> MGSDLVLGLDIGIGSVGVGILNKVTGEIIHKNSRIFPAAQAENNLVRRTNRQGRRLARRKKHRRVRLNRLFEESGLITDFTKISINLNPYQLRVKGLTDELSNEELFIALKNMVKHRGISYLDDASDDGNSSVGDYAQIVKENSKQLETKTPGQIQLERYQTYGQLRGDFTVEKDGKKHRLINVFPTSAYRSEALRILQTQQEFNPQITDEFINRYLEILTGKRKYYHGPGNEKSRTDYGRYRTSGETLDNIFGILIGKCTFYPDEFRAAKASYTAQEFNLLNDLNNLTVPTETKKLSKEQKNQIINYVKNEKAMGPAKLFKYIAKLLSCDVADIKGYRIDKSGKAEIHTFEAYRKMKTLETLDIEQMDRETLDKLAYVLTLNTEREGIQEALEHEFADGSFSQKQV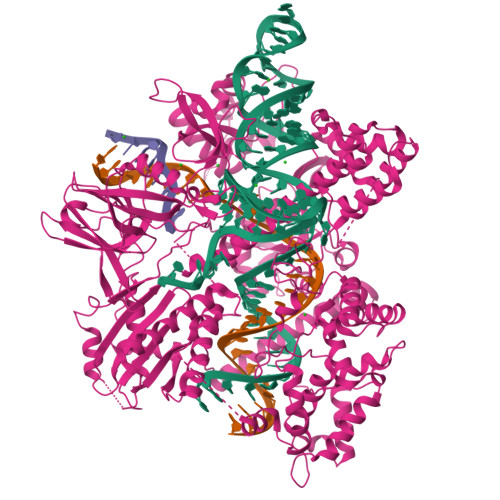DELVQFRKANSSIFGKGWHNFSVKLMMELIPELYETSEEQMTILTRLGKQKTTSSSNKTKYIDEKLLTEEIYNPVVAKSVRQAIKIVNAAIKEYGDFDNIVIEMARETNEDDEKKAIQKIQKANKDEKDAAMLKAANQYNGKAELPHSVFHGHKQLATKIRLWHQQGERCLYTGKTISIHDLINNSNQFEVDAILPLSITFDDSLANKVLVYATANQEKGQRTPYQALDSMDDAWSFRELKAFVRESKTLSNKKKEYLLTEEDISKFDVRKKFIERNLVDTRYASRVVLNALQEHFRAHKIDTKVSVVRGQFTSQLRRHWGIEKTRDTYHHHAVDALIIAASSQLNLWKKQKNTLVSYSEDQLLDIETGELISDDEYKESVFKAPYQHFVDTLKSKEFEDSILFSYQVDSKFNRKISDATIYATRQAKVGKDKADETYVLGKIKDIYTQDGYDAFMKIYKKDKSKFLMYRHDPQTFEKVIEPILENYPNKQINEKGKEVPCNPFLKYKEEHGYIRKYSKKGNGPEIKSLKYYDSKLGNHIDITPKDSNNKVVLQSVSPWRADVYFNKTTGKYEILGLKYADLQFEKGTGTYKISQEKYNDIKKKEGVDSDSEFKFTLYKNDLLLVKDTETKEQQLFRFLSRTMPKQKHYVELKPYDKQKFEGGEALIKVLGNVANSGQCKKGLGKSNISIYKVRTDVLGNQHIIKNEGDKPKLDF> GGGRPRWKRHISEQLRRRDRLQRQAFEEIILQYNKLLEKSDLHSVLAQKLQAEKHDVPNRHEISPGHDGTWNDNQLQEMAQLRIKHQEELTELHKKRGELAQLVIDLNNQMQRKDREMQMNEAKIAECLQTISDLETECLDLRTKLCDLERANQTLKDEYDALQITFTALEGKLRKTTEENQELVTRWMAEKAQEANRLNA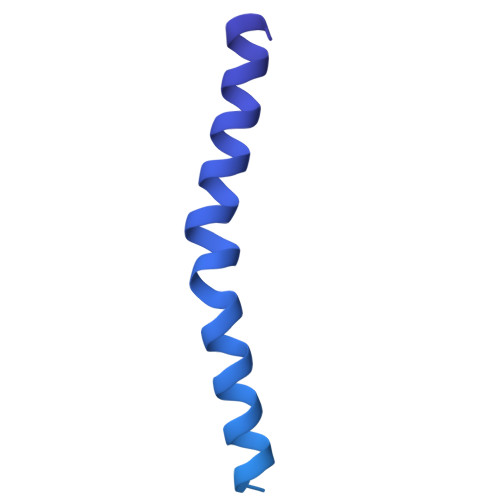ENEKDSRRRQARLQKELAEAAKEPLPVEQDDDIEVIVDETSDHTEETSPVRAISRAATKRLSQPAGGLLDSITNIFGRRSVSSFPVPQDNVDTHPGSGKE>MSLHPHLNANLEGGVLTLAIN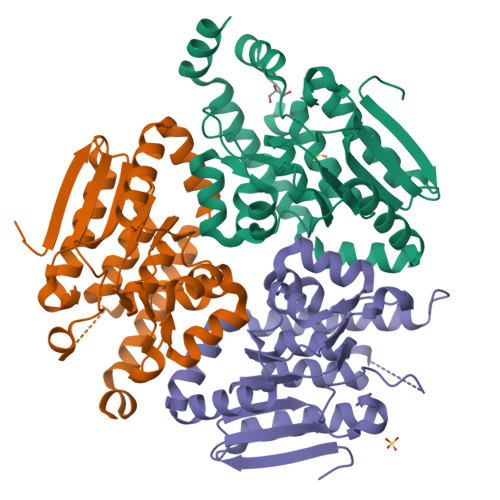RPEAKNALYGELYLWIAKALDEADQNKDVRVVVLRGAEHDFTAGNDMKDFMGFVQNPNAGPAGQVPPFVLLKSAARLSKPLIIAVKGVAIGIGVTILLQADLVFADNTALFQIPFVSLGLSPEGGASQLLVKQAGYHKAAELLFTAKKFNAETALQAGLVNEIVEDAYATAQATAQHLTALPLASLKQTKALMKHDLDQIIECIDHEAEIFMQRVQSPEMLEAVQAFMQKRQPDFSQEGHHHHHH[6x]>GAMALPSGSDPAFSQPKSVLDAGLTCQGASPSSVSKPILLVPGTGTTGPQSFDSNWIPLSAQLGYTPCWISPPPFMLNDTQVNTEYMVNAITTLYAGSGNNKLPVLTASQGGLVAQWGLTFFPSIRSKVDRLMAFAPDYKGTVLAGPLDALAVSAPSVWQQTTGSALTTALRNAGGLTQIVPTTNLYSATDEVVQPQVSNSPLDS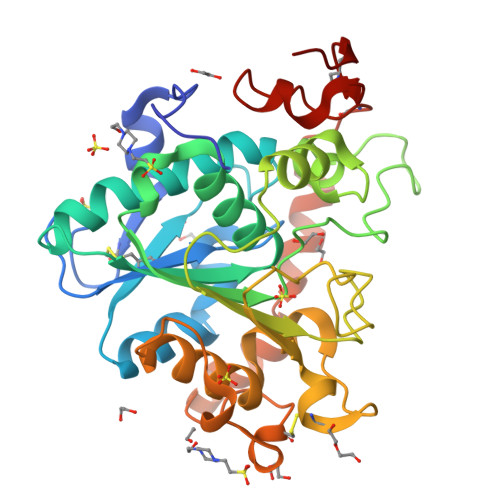SYLFNGKNVQAQAVCGPLFVIDHAGSLTSQFSYVVGRSALRSTTGQARSADYGITDCNPLPANDLTPEQKVAAAALLAPAAAAIVAGPKQNCEPDLMPYARPFAVGKRTCSGIVTP[2x]>ETKF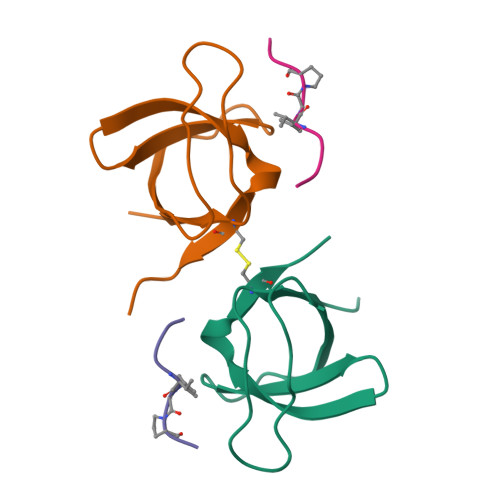VQALFDFNPQESGELAFKRGDVITLINKDDPNWWEGQLNNRRGIFPSNYVCPYNSN[2x];>XPPPVGPRR[2x]> MENTENSVDSKSIKNLEPKIIHGSESMDSGISLDNSYKMDYPEMGLCIIINNKNFHKSTGMTSRSGTDVDAANLRETFRNLKYEVRNKNDLTREEIVELMRDVSKEDHSKRSSFVCVLLSHGEEGIIFGTNGPVDLKKITNFFRGDRCRSLTGKPKLFIIQACRGTELDCGIETD;> SGVDDDMACHKIPVEADFLYAYSTAPGYYSWRNSKDGSWFIQSLCAMLKQYADKLEFMHI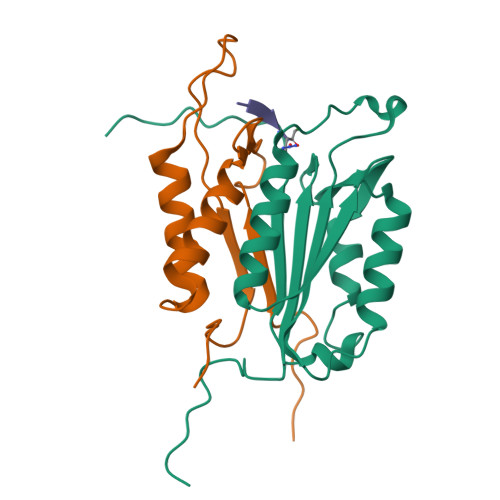LTRVNRKVADEFEDFSFDATFHAKKQIPCIVSMLTKELYFYHH> MVIDIYLKNEKEKIDFHFPVNPQDS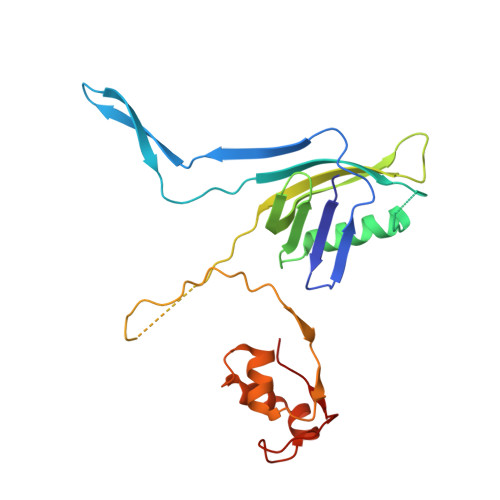LSIKKEKRFETVDIVNLGEFDIKKEGEKIREISFKTFLPNLYDASYCRYSELKNPIEVVAMLEKWVDQAEPLRLIITGFGYNGLVTISSFSNTQTAGREEDRDIEITFRTYRELKIETLKKDTKSNTKTDLKDNRPNTQTKSKIYTVKASDTLYKIAKNLLGKGSRWPEIYNIPENKKVIGKNPNIIKKGQKLVIPSK>[6x]MKLIDKLPSFDRNYIVEEIQGAYDTELNILKEDIDDTFNQLFVDTATWGLDMWEDILCIEKKELDFDTRRSNIKAKMRSRGTSTIEVIKSICEAYTKSETDIKVYSDEFTFVLSFIANNCDYKTLLDCSDMIERVKPAHLLHYLEPIILDKSMVYCGGGMVCSEEVKVHPYFEPIIKCSAVVNCGAGMISREEIKVYPLSIKCIENNCKINIAIANDTGVENVVVYPKSEVV;>MYSDQTYEVIKNRTLENINLDIYKGEGSFLNNMVSGNNLELSKIYLELSKMHKMAFIQDTYNQFLDKRVNEFGVYRKLGTESNGEVEFIGEKGTVINNGTIISYRDLLFVVIKDVTIGSEEGDNSPVQALEVGKKYNLPTNCEFKLVDNISGVTKITNTRSFEGGTDIETDEELKERFYKIQRNQATSGNKAHYEEWALEVDGVYNVKVYPRWDGPGTVKVLIFGKNNQAVDTETIERCQQHIDEEKPIGPTITVVTPLPIEISISAVMKLEDGYTLDNVKESFLESINTYFRDIRGEIIYTKVMGILINTTGVHDLSNLLINGSTDNITINEDKIPSVTTVNFSEVENQ[12x];>MAIGLPSINISFKELATTVKERSARGIIAMVLKDAKALGLNEIHEKEDIPVDLSAENKEYINLALMGNVNTPNKLLVYVIEGEADIQTALDFLETKEFNYLCMPKAVEADKTAIKNWIIKLRDIDKVKVKAVLGKVVGNHEGIINFTTEDVLVGEKKYSVDEFTSRVAGLIAGTPLSQSVTYTKLSDVVDIPKMTKVDAESRVNKGELILIKEAGAIRIARGVNSLTELTAEKGEMFQKIKIVDTLDIIHSDIRKVIIDDYIGKVTNSYDNKCLLIVAIKSYLEELEKSALIESDSTVEIDFEAQKSYLKSKGVDLSYMTLQEIKEANTGSKVFLKAKIKVLDAMEDIDLSIEI[18x];>[6x]MSTIFPFI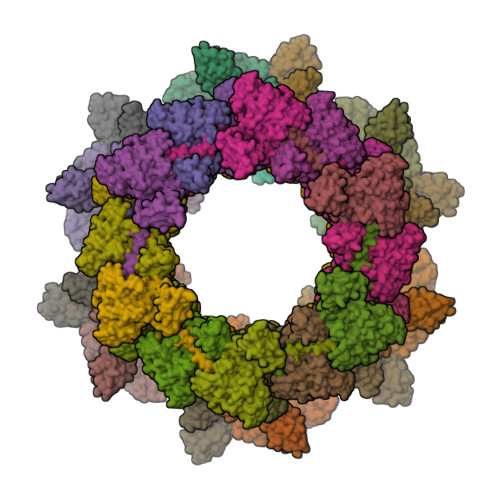GVPEDYILPKTEELPIFREVAWDFEKDEPILEKGDFKIIEKKEALKVWIYKCIKTNRYEHEIYSLEYGTELSELIGQKYTKGLTESEASRFIKEALLINPYILEVNVKSANFNRDILSANVKVSTIYGEVEINV>[2x]SETSRTAFGGRRAVPPNNSNAAED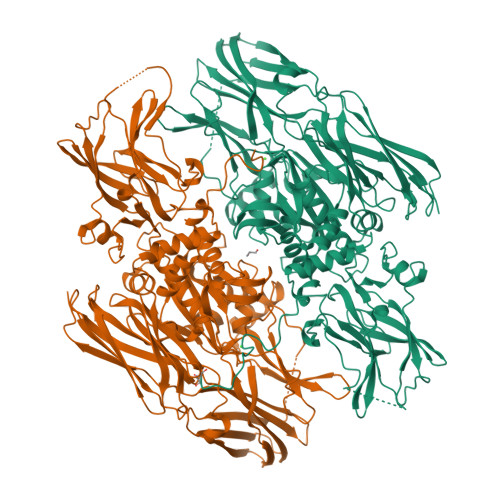DLPTVELQGVVPRGVNLQEFLNVTSVHLFKERWDTNKVDHHTDKYENNKLIVRRGQSFYVQIDFSRPYDPRRDLFRVEYVIGRYPQENKGTYIPVPIVSELQSGKWGAKIVMREDRSVRLSIQSSPKCIVGKFRMYVAVWTPYGVLRTSRNPETDTYILFNPWCEDDAVYLDNEKEREEYVLNDIGVIFYGEVNDIKTRSWSYGQFEDGILDTCLYVMDRAQMDLSGRGNPIKVSRVGSAMVNAKDDEGVLVGSWDNIYAYGVPPSAWTGSVDILLEYRSSENPVRYGQCWVFAGVFNTFLRCLGIPARIVTNYFSAHDNDANLQMDIFLEEDGNVNSKLTKDSVWNYHCWNEAWMTRPDLPVGFGGWQAVDSTPQENSDGMYRCGPASVQAIKHGHVCFQFDAPFVFAEVNSDLIYITAKKDGTHVVENVDATHIGKLIVTKQIGGDGMMDITDTYKFQEGQEEERLALETALMYGAKKPLNTEGVMKSRSNVDMDFEVENAVLGKDFKLSITFRNNSHNRYTITAYLSANITFYTGVPKAEFKKETFDVTLEPLSFKKEAVLIQAGEYMGQLLEQASLHFFVTARINETRDVLAKQKSTVLTIPEIIIKVRGTQVVGSDMTVTVQFTNPLKETLRNVWVHLDGPGVTRPMKKMFREIRPNSTVQWEEVCRPWVSGHRKLIASMSSDSLRHVYGELDVQIQRRPSM>[6x]MLRTMLKSKIHRATVTCADLHYVG;>XVTIDADLMDAADLLEGEQVTIVDIDNGARLVTYAITGERGSGVIGINGAAAHLVHPGDLVILIAYATMDDARARTYQPRIVFVDAYNKPIDMGHDPAFVPENAGELLDPRLGVGLEHHHHHH[6x]

Here, we present biochemical and structural evidence that POA inhibits Mtb PanD in a competitive fashion and that it binds with a high degree of complementarity to the active site of the enzyme. PanD is a proenzyme and in the structure, we observed the processed active enzyme after cleavage between Gly24 and Ser25, and modification of Ser25 to a pyruvoyl group (Pyr25). The active protein consists of a β chain (Met1-Gly24) and an α chain (Pyr25 to ILE115). Our results show that resistance to PZA in PanD mutants primarily comes from alterations in two loops covering the active site that have subtle, but significant effects on the affinity and residence time of POA on the enzyme rather than from directly affecting POA binding interactions.

The crystal structures of apo Mtb PanD and the Mtb PanD:POA complex were solved using molecular replacement and both structures were refined to 2.7 Å resolution. In the POA complex structure, there was one molecule of POA bound to each Mtb PanD active site, which was located at the interface between two adjacent subunits of the PanD tetramer. The density for POA was clearly visible in a difference electron density map made by subtracting the structure factor amplitudes of the apo crystal diffraction data from that of the PanD:POA complex, as well as a polder OMIT map. Because of the internal symmetry of the POA there are two ways to fit POA to the electron density. We choose to position the molecule based on optimal hydrogen bonding. There were four hydrogen bonds that contribute significantly to the binding between POA and PanD: two between POAs carboxylate oxygens and the amide groups on the backbone of Ala74 (2.7 Å) and Ala75 (2.7 Å), one between a carboxylate oxygen to the guanidinium group of Arg54* (2.8 Å), and another between the N1 on the POA pyrazine ring and Arg54* (2.9 Å). Thus, POA binds to the active site of Mtb PanD interacting with the same groups as the substrate, and this is consistent with a competitive mode of inhibition. The POA binding pocket is relatively small (206 Å3) and not easily accessible, as there is only a narrow tunnel leading from the active site to the inside barrel of the PanD tetramer. While we cannot be certain through which portal the substrate or inhibitor enters the active site, the protein must undergo a significant conformational change to allow substrate or POA access to the active site. This conformational change requirement for binding of molecules to the active site may account for the slow on- and off-rate of POA binding.> XRMKQIEDKIEEIESKQKK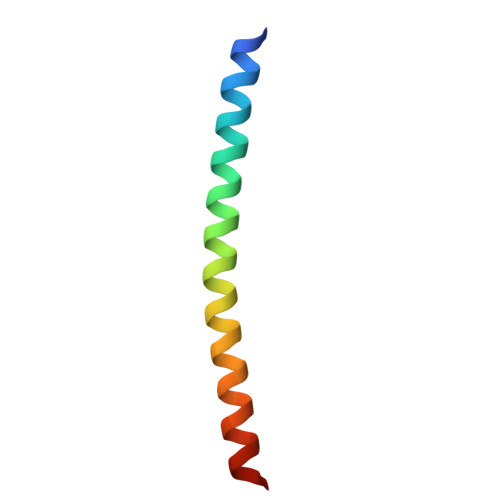IENEIARIKKLLQLTVWGIKQLQARILX>MWELTILHTNDVHSRLEQTSEDSSKCVDASRCMGGVARLFTKVQQIRRAEPNVLLLDAGDQYQGTIWFTVYKGAEVAHFMNALRYDAMALGNHEFDNGVEGLIEPLLKEAKFPILSANIKAKGPLASQISGLYLPYKVLPVGDEVVGIVGYTSKETPFLS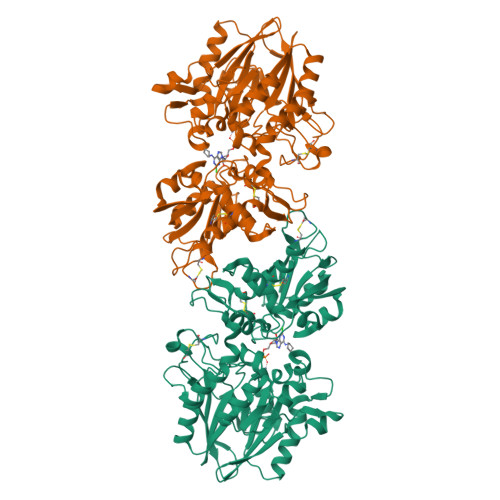NPGTNLVFEDEITALQPEVDKLKTLNVNKIIALGHSGFEMDKLIAQKVRGVDVVVGGHSNTFLYTGNPPSKEVPAGKYPFIVTSDDGRKVPVVQAYAFGKYLGYLKIEFDERGNVISSHGNPILLDSSIPEDPSIKADINKWRIKLDDYSTQELGKTIVYLDGSSQSCRFRECNMGNLICDAMINNNLRHADEMFWNHVSMCILNGGGIRSPIDERNDGTITWENLAAVLPFGGTFDLVQLKGSTLKKAFEHSVHRYGQSTGEFLQVGGIHVVYDLSRKPGDRVVKLDVLCTKCRVPSYDPLKMDEVYKVILPNFLANGGDGFQMIKDELLRHDSGDQDINVVSTYISKMKVIYPAVEGRIKFSLEHHHHHH[2x]> NPVENYIDEVLNEVLVVPNINSSNPTTSNSAPALDAAETGHTSSVQPEDVIETRYVQTSQTRDEMSLESFLGRSGCIHESKLEVTLANYNKENFTVWAINLQEMAQIRRKFELFTYTRFDSEITLVPCIS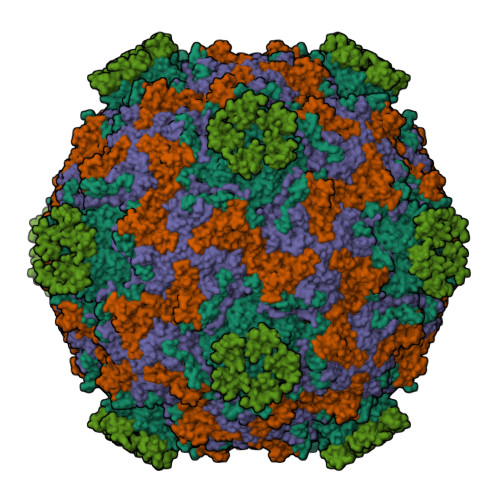ALSQDIGHITMQYMYVPPGAPVPNSRDDYAWQSGTNASVFWQHGQAYPRFSLPFLSVASAYYMFYDGYDEQDQNYGTANTNNMGSLCSRIVTEKHIHKVHIMTRIYHKAKHVKAWCPRPPRALEYTRAHRTNFKIEDRSIQTAIVTRPIITTAGPSDMY;> SPTVEACGYSDRIIQITRGDSTITSQDVANAIVAYGVWPHYLSSKDASAIDKPSQPDTSSNRFYTLRSVTWSSSSKGWWWKLPDALKDMGIFGENMFYHYLGRSGYTIHVQCNASKFHQGTLIVALIPEHQIASALHGNVNVGYNYTHPGETGREVKAETRLNPDLQPTEEYWLNFDGTLLGNITIFPHQFINLRSNNSATIIAPYVNAVPMDSMRSHNNWSLVIIPICPLETSSAINTIPITISISPMCAEFSGARAKRQ;> GLPVFITPGSGQFLTTDDFQSPCALPWYHPTKEISIPGEVKNLVEICQVDSLVPINNTDTYINSENMYSVVLQSSINAPDKIFSIRTDVASQPLATTLIGEISSYFTHWTGSLRFSFMFCGTANTTVKLLLAYTPPGIAEPTTRKDAMLGTHVIWDVGLQSTISMVVPWISASHYRNTSPGRSTSGYITCWYQTRLVIPPQTPPTARLLCFVSGCKDFCLRMARDTNLHLQSGAIAQ;> GAQVSRQNVGTHSTQNSVSNGSSLNYFNINYFKDAASNGASKLEFTQDPSKFTDPVKDVLEKGIPTLQ;> RTCRIHEISCGAHSTQCIPVSWRCDGENDCDSGEDEENCGN> GQANHPTAAVVTEKQQMLEQHLQDVRKRVQDLEQKMKVVENLQDDFDFNYKTLKSQGDMQDLNGNNQSVTRQKMQQLEQMLTALDQMRRSIVSELAGLLSAMEYVQKTLTDEELADWKRRQQIACIGGPPNICLDRLENWITSLAESQLQTRQQIKKLEELQQKVSYKGDPIVQHRPMLEERIVELFRNLMKSAFVVERQPCMPMHPDRPLVIKTGVQFTTKVRLLVKFPELNYQLKIKVCIDKDSGDVAALRGSRKFNILGTNTKVMNMEESNNGSLSAEFKHLTLREQRCGNGGRANCDASLIVTEELHLITFETEVYHQGLKIDLETHSLPVVVISNICQMPNAWASILWYNMLTNNPKNVNFFTKPPIGTWDQVAEVLSWQFSSTTKRGLSIEQLTTLAEKLLGPGVNYSGCQITWAKFCKENMAGKGFSFWVWLDNIIDLVKKYILALWNEGYIMGFISKERERAI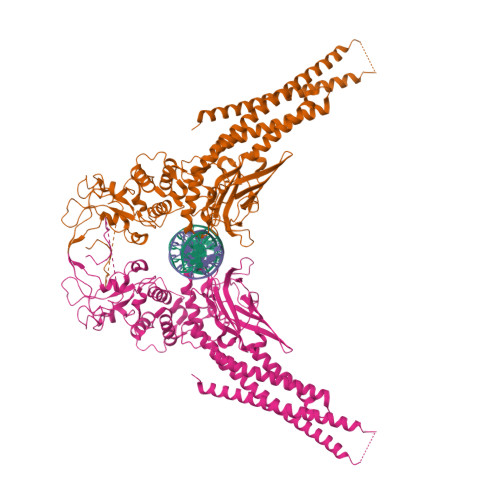LSTKPPGTFLLRFSESSKEGGVTFTWVEKDISGSTQIQSVEPYTKQQLNNMSFAEIIMGYKIMDATNILVSPLVYLYPDIPKEEAFGKYCRPESQEHPEADPGSAAPYLKTKFICVTPFIDAVWK> KLLPAFQNAERLLLAHMMRSRDVALVVQERIGGRFNIEEHRALAAYIYAFYEEGHEADPGALISRIPGELQPLASELSLLLIADDVSEQELEDYIRHVLNRPKWLMLKVKEQEKTEAERR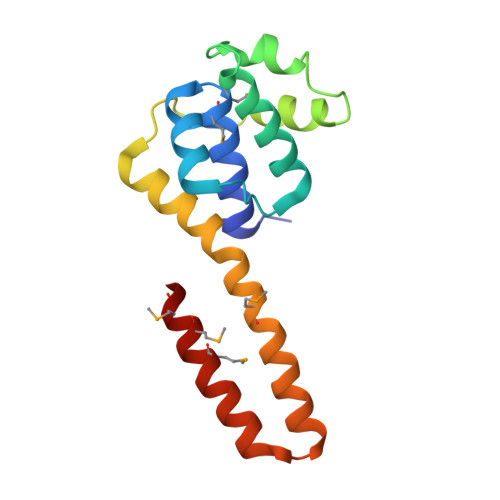KDFLTAARIAKEMIEMKKMLSSS> GAMDTTYLTEEVKRGNIEKNVVATGSIESINTVDVGAQVSGKITKLYVKLGQQVKKGDLLAEIDSTTQINTLNTRKAALASYQAQLVARKTAYDVALSNYQRLSKLYGQKA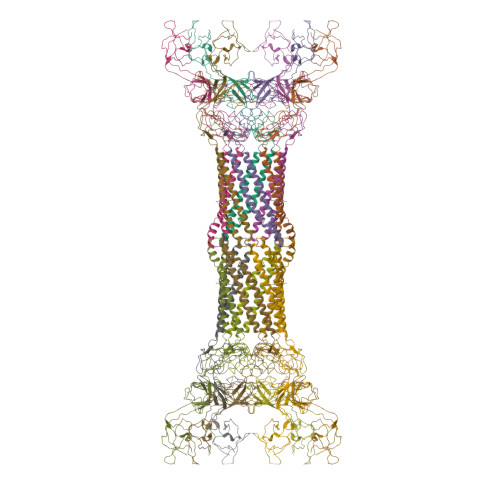TSLDTLNTAKATLNNAKAEMDVVQENIKQAEIEVNTAETNLGYTKITSPIDGTVISTPVSEGQTVNSNQTTPTIIKVADLSKMRIKPEISEGDITKVKAGQDVTFTILSDNKTVYHAKIDSVDPATTTISDNSSSNSSSSGSSSSSGSSSSAVYYYANIIVENPEHVLRIGMTTENNIKIADVQNVLFIPNLAVQKQQDKYVVNVLNGNTTQEREIEIGVQNDFQTEVKSGLTEGEKVVISQVAAGETFGDPDAPIIF> MDYIKGIAFDLYGTLFDVHSVVGRCDEAFPGRGREISALWRQKQLEYTWLRSLMNRYVNFQQATEDALRFTCRHLGLDLDARTRSTLCDAYL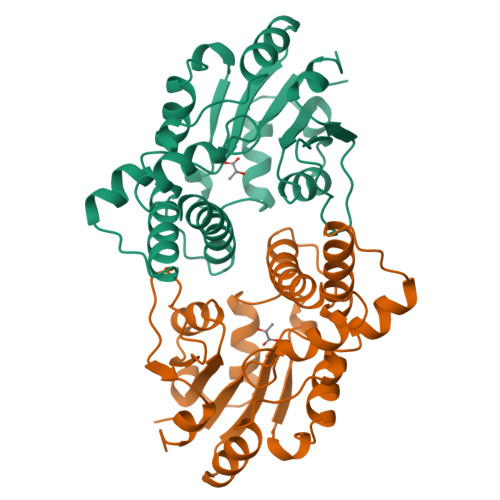RLAPFSEVPDSLRELKRRGLKLAILSNGSPQSIDAVVSHAGLRDGFDHLLSVDPVQVYKPDNRVYELAEQALGLDRSAILFVSSNAWDATGARYFGFPTCWINRTGNVFEEMGQTPDWEVTSLRAVVELFETAAGKAEKG>[4x]MVPAESNAVQAKLAKTLQRFENKIKAGDYYEAHQTLRTIANRYVRSKSYEHAIELISQGALSFLKAKQGGSGTDLIFYLLEVYDLAEVKVDDISVARLVRLIAELDPSEPNLKDVITGMNN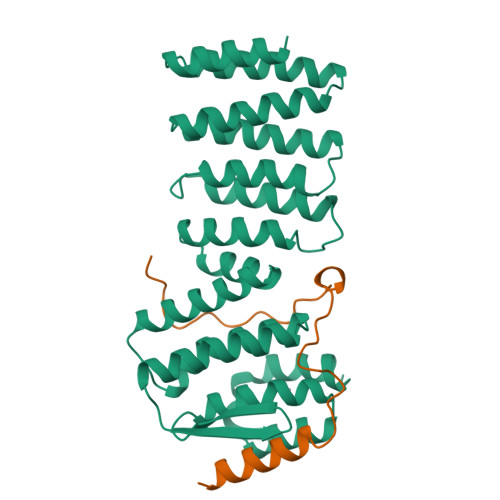WSIKFSEYKFGDPYLHNTIGSKLLEGDFVYEAERYFMLGTHDSMIKYVDLLWDWLCQVDDIEDSTVAEFFSRLVFNYLFISNISFAHESKDIFLERFIEKFHPKYEKIDKNGYEIVFFEDYSDLNFLQLLLITCQTKDKSYFLNLKNHYLDFSQAYKSELEFLGQEYFNIVAPKQTNFLQDMMSGFLGGSK;>MSTSASGPEHEFVSKFLTLATLTEPKLPKSYTKPLKDVTNLGVPLPTLKYKYKQNRAKK[4x]4-(hydroxymethyl)-1-(alpha-D-mannopyranosyl)-1H-1,2,3-triazole | C9 H15 N3 O6 | 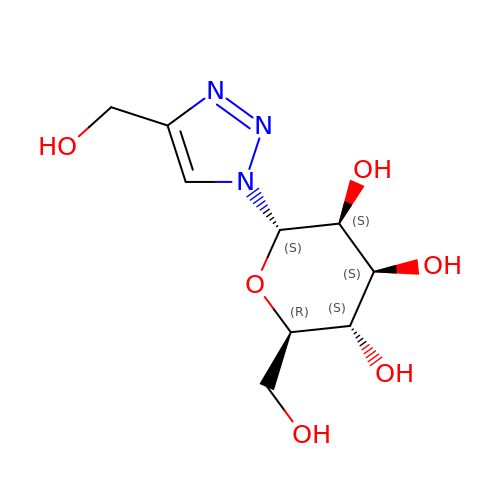BHGZOVXPACYZLI-DFTQBPQZSA-N>[2x]MSMSDINKNSELIFIPAPGIGHLASALEFAKLLTNHDKNLYITVFCIKFPGMPFADSYIKSVLASQPQIQLIDLPEVEPPPQELLKSPEFYILTFLESLIPHVKATIKTILSNKVVGLVLDFFCVSMIDVGNEFGIPSYLFLTSNVGFLSLMLSLKNRQIEEVFDDSDRDHQLLNIPGISNQVPSNVLPDACFNKDGGYIAYYKLAERFRDTKGIIVNT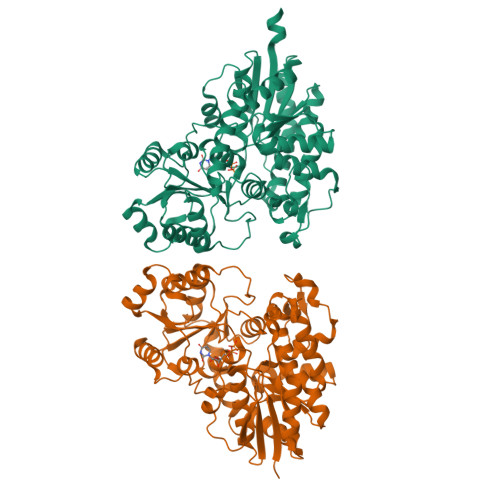FSDLEQSSIDALYDHDEKIPPIYAVGPLLDLKGQPNPKLDQAQHDLILKWLDEQPDKSVVFLCFGSMGVSFGPSQIREIALGLKHSGVRFLWSNSAEKKVFPEGFLEWMELEGKGMICGWAPQVEVLAHKAIGGFVSHCGWNSILESMWFGVPILTWPIYAEQQLNAFRLVKEWGVGLGLRVDYRKGSDVVAAEEIEKGLKDLMDKDSIVHKKVQEMKEMSRNAVVDGGSSLISVGKLIDDITG>[4x]SPQSKSRKIAILGYRSVGKSSLTIQFVEGQFVDSYDPTIENTFTKLITVNGQEYHLQLVDTAGQDEYSIFPQTYSIDINGYILVYSVTSIKSFEVIKVIHGKLLDMVGKVQIPIMLVGNKKDLHMERVISYEEGKALAESWNAAFLESSAKENQTAVDVFRRIILEAEKLE

Growth factor signaling into mTORC1 is regulated by the heterotrimeric TSC complex, which acts as a GTPase-activating protein (GAP) for Ras homolog enriched in brain (Rheb), a GTP-binding protein that is broadly expressed in human and mammalian tissues. Rheb is a monomeric protein with a molecular weight of about 21 kDa. As in the closely related small GTPase Ras, the flexible switch I region of Rheb undergoes a conformational change during nucleotide hydrolysis and exchange, while the switch II region remains largely unchanged. Point mutations in the switch II region of Rheb (Y67A/I69A and I76A/D77A) impair its ability to activate mTORC123, implying that the switch II region is key to Rheb’s function in mTORC1 activation.

Crystal structures of GDP- and GTP-bound Rheb have been reported, and the switch II domain is typically disordered and adopts different conformations. We obtained a 2.05 Å structure of GDP-bound Rheb and replicated the results reported by Yu et al.. 1 was then soaked into the same crystals, whereupon additional electron density was observed in the switch II domain.N-(5-chloro-1,3-benzodioxol-4-yl)-6-methoxy-7-(3-piperidin-1-ylpropoxy)quinazolin-4-amine 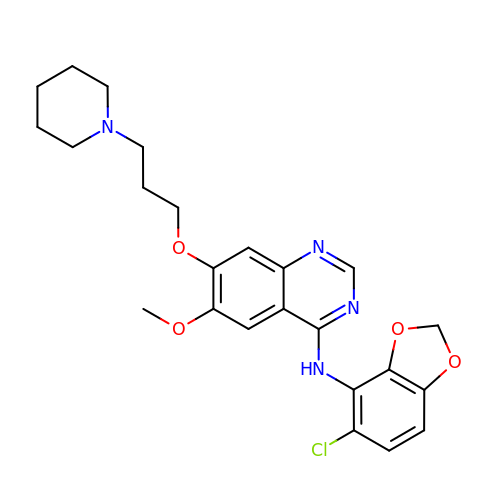| C24 H27 Cl N4 O4 | QHIMVPIOWKYPSO-UHFFFAOYSA-N>MDFGSLETVVANSAFIAARGSFDASSGPASRDRKYLARLKLPPLSKCEALRESLDLGFEGMCLEQPIGKRLFQQFLRTHEQHGPALQLWKDIEDYDTADDALRPQKAQALRAAYLEPQAQLFCSFLDAETVARARAGAGDGLFQPLLRAVLAHLGQAPFQEFLDSLYFLRFLQWKWLEAQPMGEDWFLDFRVLGRGGFGEVFACQMKATGKLYACKKLNKKRLKKRKGYQGAMVEKKILAKVHSRFIVSLAYAFETKTDLCLVMTIMNGGDIRYHIYNVDEDNPGFQEPRAIFYTAQIVSGLEHLHQRNIIYRDLKPENVLLDDDGNVRISDLGLAVELKAGQTKTKGYAGTPGFMAPELLLGEEYDFSVDYFALGVTLYEMIAARGPFRARGEKVENKELKQRVLEQAVTYPDKFSPASKDFCEALLQKDPEKRLGFRDGSCDGLRTHPLFRDISWRQLEAGMLTPPFVPD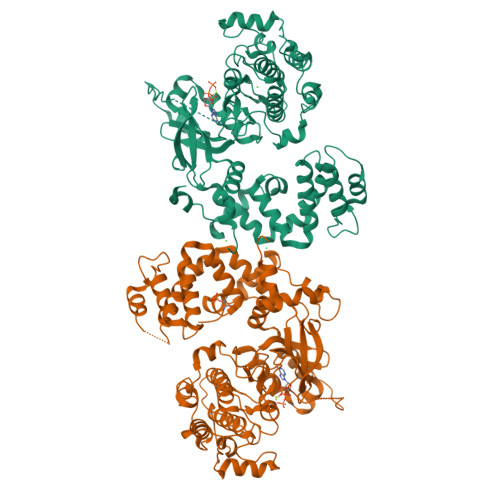SRTVYAKNIQDVGAFSTVKGVAFEKADTEFFQEFASGTCPIPWQEEMIETGVFGDLNVWRPDGVDHHHHHH[2x]>[2x]IIKIIK

High expression of PSMαs, which are four peptides of about 20-residues in length, increases virulence potential of methicillin-resistant S. aureus (MRSA). Amyloid aggregation plays roles in PSM activities in S. aureus. In the present study, we investigated the structure-function relationships of PSMαs and their short truncations.

To obtain atomic-level insights into the architecture of PSMα1 and PSMα4 fibrils, we computationally identified their amyloidogenic spine segments, and determined their high-resolution structures by means of X-ray microcrystallography. Segments PSMα1-IIKVIK and PSMα4-IIKIIK, both of which are conserved within naturally occurring PSM truncations, adopt the canonical cross-β fibril architecture, wherein pairs of β-sheets tightly mate through a dry interface, forming a steric zipper. Both structures belong to the class 1 of steric zippers, indicating that parallel β-sheets mate face-to-face in the fibrils formed by the PSMα1-IIKVIK and PSMα4-IIKIIK segments. Proline substitutions in these spine regions abolished fibril formation of the full-length PSMα1 and PSMα4. Structural indicators of fibril stability of the IIKVIK and IIKIIK segments, i.e., buried surface area and shape complementarity between sheets, calculated from the crystal structures, resemble those of eukaryotic steric-zipper structures. The contrasting levels of stability of PSMα3-LFKFFK and PSMα4-IIKIIK fibrils, inferred from structural analyses, were verified experimentally. Specifically, PSMα3-LFKFFK fibrils dissolve upon heating to 50 °C, and reform upon cooling, whereas PSMα4-IIKIIK fibrils remain stable. While PSMα3 forms cross-α fibrils and enhances toxicity against human cells, PSMα1 and PSMα4 form cross-β fibrils which likely play a role in stabilizing the biofilm matrix. The highly stable steric zipper structures, forming the spines of the cross-β fibrils, putatively serve as the building block cementing the biofilm and creating the rigidity that can explain the resistance of amyloid-containing biofilms. The atomic structures of the PSMα1 and PSMα4 derivatives offer templates for the design of anti-biofilm compounds.>HHGGEHFEGEKVFRVNVEDENHINIIRELASTTQIDFWKPDSVTQIKPHSTVDFRVKAEDTVT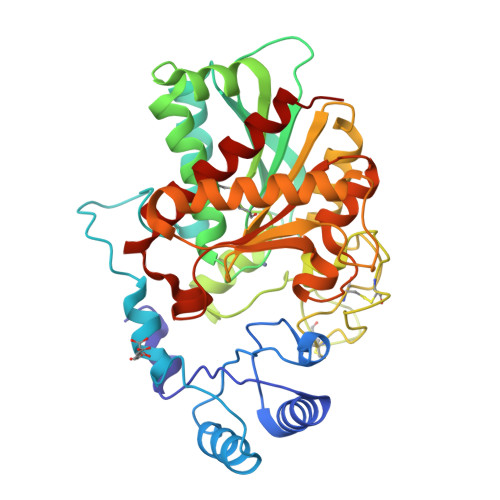VENVLKQNELQYKVLISNLRNVVEAQFDSRVRATGHSYEKYNKWETIEAWTQQVATENPALISRSVIGTTFEGRAIYLLKVGKAGQNKPAIFMDCGFHAREWISPAFCQWFVREAVRTYGREIQVTELLNKLDFYVLPVLNIDGYIYTWTKSRFWRKTRSTHTGSSCIGTDPNRNFDAGWCEIGASRNPCDETYCGPAAESEKETKALADFIRNKLSSIKAYLTIHSYSQMMIYPYSYAYKLGENNAELNALAKATVKELASLHGTKYTYGPGATTIYPAAGGSDDWAYDQGIRYSFTFELRDTGRYGFLLPESQIRATCEETFLAIKYVASYVLEHLY[2x]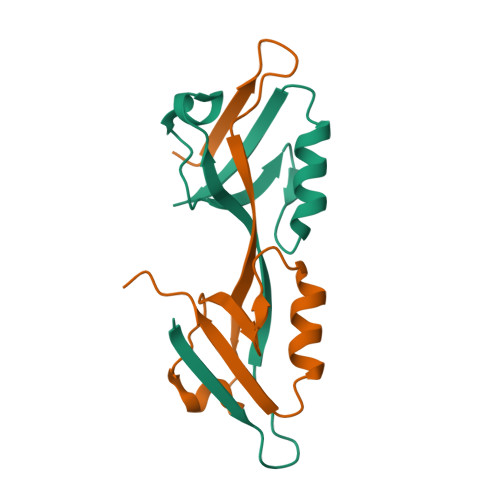>GSKVTLVKSRKNEEYGLRLASHIFVKEISQDSLAARDGNIQEGDVVLKINGTVTENMSLTDAKTLIERSKGKLKMVVQRDE[2x]>GVALGATRVIYPAGQKQEQLAVTNNDENSTYLIQSWVENADGVKDGRFIVTPPLFAMKGKKENTLRILDATNNQLPQDRESLFWMNVKAIPSMDKSKLT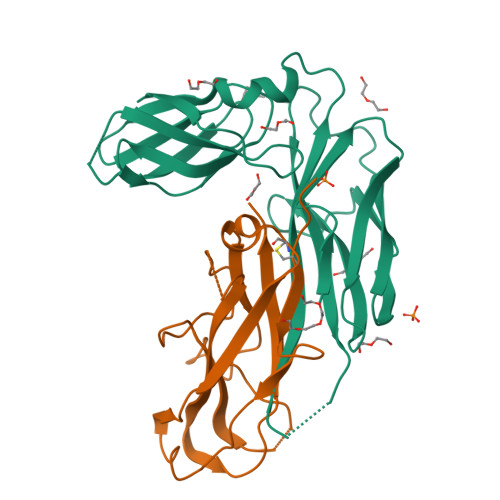ENTLQLAIISRIKLYYRPAKLALPPDQAAEKLRFRRSANSLTLINPTPYYLTVTELNAGTRVLENALVPPMGESTVKLPSDAGSNITYRTINDYGALTPKMTGVME[2x];>[2x]MNAACAVDAGSVDQTVQLGQVRTASLAQEGATSSAVGFNIQLNDCDTNVASKAAVAFLGTAIDAGHTNVLALQSSAAGSATNVGVQILDRTGAALTLDGATFSSETTLNNGTNTIPFQARYFATGAATPGAANADATFKVQYQ NEOAGAROBIOSE 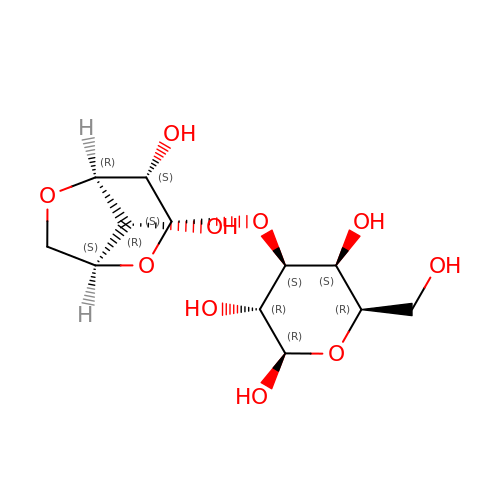| C12 H20 O10 | JWMBOBQNPBCYER-AHBMTURSSA-N>[8x]SNAKHDVFPSFHGADVRRTFLSHILESFRRKGIDTFIDNNIERSKSIGPELKEAI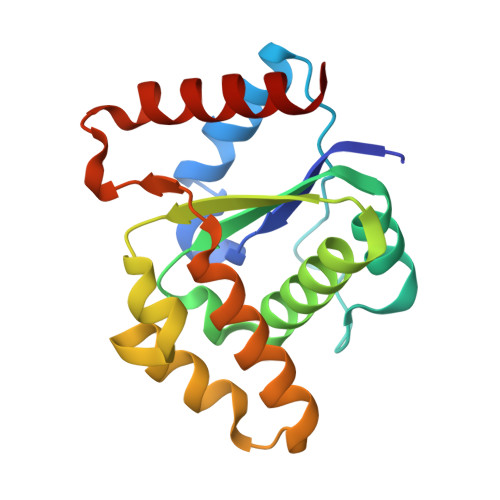KGSKIAIVLLSRKYASSSWCLDELAEIMICREVLGQIVMTIFYEVDPTDIKKQTGEFGKAFTKTCRGKPKEQVERWRKALEDVATIAGYHSHKWCDEAEMIEKISTDVSNMLD>MVLYFIGLGLYDERDITVKGLEIAKKCDMVFAEFYTSLMAGTTLGRIQKLIGKEIRVLSREDVELNFENIVLPLAKENDVAFLTPGDPLVATTHAELRIRAKRAGVESYVIHAPSIYSAVGITGLHIYKFGKSATVAYPEGNWFPTSYY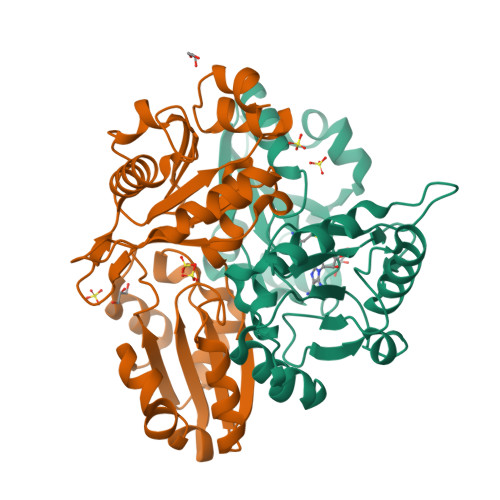DVIKENAERGLHTLLFLDIKAEKRMYMTANEAMELLLKVEDMKKGGVFTDDTLVVVLARAGSLNPTIRAGYVKDLIREDFGDPPHILIVPGKLHIVEAEYLVEIAGAPREILRVNV[2x]> MPTEFLYTSKIAAISWAATGGRQQRVYFQDLNGKIREAQRGGDNPWTGGSSQNVIGEAKLFSPLAAVTWKSAQGIQIRVYCVNKDNILSEFVYDGSKWITGQLGSVGVKVGSNSKLAALQWGGSESAPPNIRVYYQKSNGSGSSIHEYVWSGKWTAGASFGSTVPGTGIGATAIGPGRLRIYYQATDNKIREHCWDSNSWYVGGFSASASAGVSIAAISWGSTPQIRVYWQKGREELYEAAYGGSWNTPGQIKDASRPTPSLPDTFIAANSSGNIDISVFFQASGVSLQQWQWISGKGWSIGAVVPTGTPAGWLEHHHHHHHHHH

Lectins are carbohydrate-binding proteins that are widely used in medicinal research for lectin-staining of cells and tissues as well as for glycoprotein analysis. One of the predominantly used lectins is AAL from Aleuria aurantia—the first fungal lectin with a solved 3D structure. It combines high affinity towards fucose and fucosylated oligosaccharides with an ability to recognize core fucosylated oligosaccharides with α1–6 linked fucose. There are five slightly different binding sites per AAL monomer and there is evidence for the presence of at least one so called high-affinity binding site.

In this study, we present the high resolution X-ray structure of the AALN224Q lectin complex with α-methyl-l-fucoside where the Trp side chain is found in both conformations. The protein adopts the 6-bladed β-propeller fold highly similar to a previously determined structure of the AAL/Fuc complex. The structure contains a monomeric unit of the lectin bound to α-methyl-l-fucoside residue (αMeFuc) in all five binding sites. All five binding sites are very similar and the main difference among them is that three of them contain the Trp residue which creates CH-π stacking interaction with bound Fuc residue, whereas the remaining two binding sites contain the Tyr residue which also creates CH-π interaction. The single point mutation N224Q reported previously to affect the binding affinity of site 5 is not directly involved in ligand binding. Analysing the high resolution structure of Aleuria aurantia lectin AAL in complex with αMeFuc, we identified CH–π interacting Trp residue being present in two conformations with the same occupancy in binding Site2 and Site5, while only one conformation is preferred in Site3. In binding Site3, where CH-π interaction is also mediated by tryptophan residue (Trp194), only g(‒) conformation was found. This is stabilized by a water molecule bridge between NE1 of Trp194 and the backbone O of Gly176. The hydrogen bond network of the αMeFuc is not affected by the Trp conformation within any of the binding sites. The observed Eint suggest that both stacking Trp conformations are equivalent in strength even though they create slightly different interactions with αMeFuc.> MSLTRPLRADAARNRARVLEVAYDTFAAEGLGVPMDEIARRAGVGAGTVYRHFPTKQALVVAVAEDRVRRIVDHARTLLAAEGPGEALFVFMRDM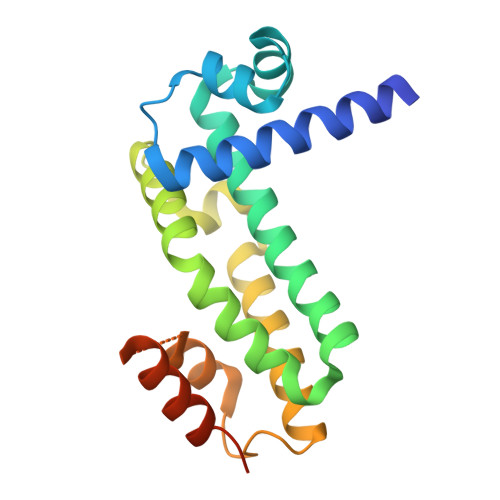VRSAAADYGLVDALVGYGLDLEVAAPGAEAAFLATLGELLAAAQRAGTVRADVDVAVIKALLVVCKVPQVYDGEVSERVVRVIEDGLRVRSSVEGHHHHHH> FQQLSARLQEAIGRLRGRGRITEEDLKATLREIRRALMDADVNLEVTRDFVERVREEALGKQVLESLTPAEVILATVYEALKEALGGEARLPVLKDRNLWFLVGLQGSG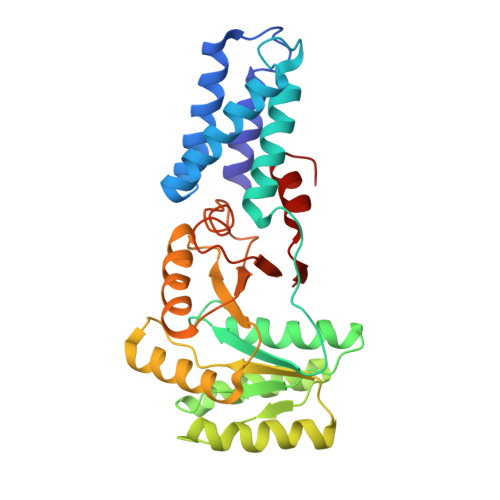KTTTAAKLALYYKGKGRRPLLVAADTQRPAAREQLRLLGEKVGVPVLEVMDGESPESIRRRVEEKARLEARDLILVDTAGRLQIDEPLMGELARLKEVLGPDEVLLVLDAMTGQEALSVARAFDEKVGVTGLVLTKLDGDARGGAALSARHVTGKPIYFAGVSEKPEGLEPFYPERLAGRILGMG> MKLERVTVKNFRSHSDTVVEFKEGINLIIGQNGSGKSSLLDAILVGLYWPLRIKDIKKDEFTKVGA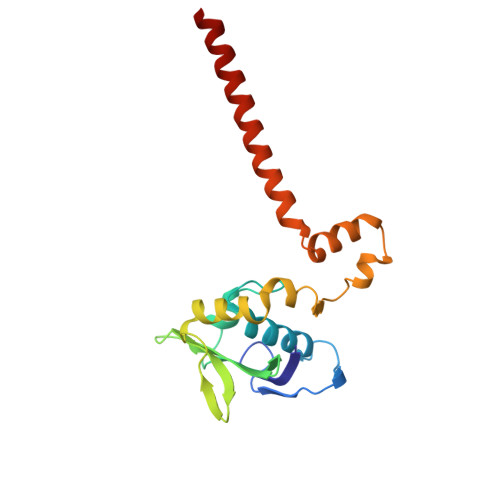RDTYIDLIFEKDGTKYRITRRFLKGYSSGEIHAMKRLVGNEWKHVTEPSSKAISAFMEKLIPYNIFLNAIYIRQGQIDAILESDEAREKVVREVLNLDKFETAYKKLSELKKTINNRIKEYRDILARTE> APIRVVSVPESDSFMSSVPDNSTPLYPKVVVPPRQVPGRFTNFIDVAKQTYSFCSISGKPYFEVTNTSGDE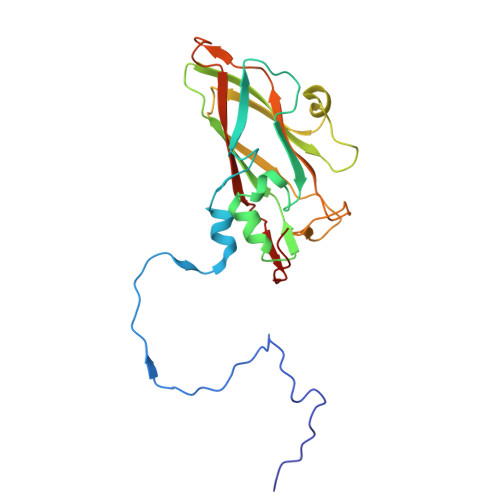PLFQMDVSLSAAELHGTYVASLSSFFAQYRGSLNFYFIFTGAAATKAKFLVAFVPPHSAAPKTRDEAMACIHAVWDVGLNSAFSFNVPYSSPADFMAVYSAEATVVNVSGWLQVYALTALTSTDIAVNSKGRVLVAVSAGPDFSLRHPVDLPDKQ>[8x]MNNMNVIIADDHPIVLFGIRKSLEQIEWVNVVGEFEDSTAL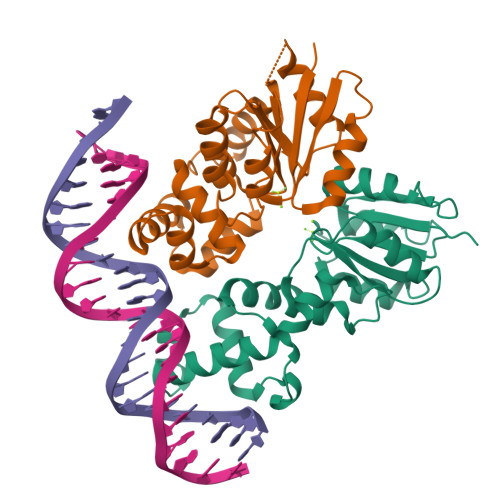INNLPKLDAHVLITDLSMPGDKYGDGITLIKYIKRHFPSLSIIVLTMNNNPAILSAVLDLDIEGIVLKQGAPTDLPKALAALQKGKKFTPESVSRLLEKISAGGYGDKRLSPKESEVLRLFAEGFLVTEIAKKLNRSIKTISSQKKSAMMKLGVENDIALLNYLSSVTLSPTDKE> MVHLGPKKPQARKGSMADVPKELMDEIHQLEDMFTVDSETLRKVVKHFIDELNKGLTKKGGNIPMIPGWVMEFPTGKESGNYLAIDLGGTNLRVVLVKLSGNHTFDTTQSKYKLPHDMRTTKHQEELWSFIADSLKDFMVEQELLNTKDTLPLGFTFSYPASQNKINEGILQRWTKGFDIPNVEGHDVVPLLQNEISKRELPIEIVALINDTVGTLIASYYTDPETKMGVIFGTGVNGAFYDVVSDIEKLEGKLADDIPSNSPMAINCEYGSFDNEHLVLPRTKYDVAVDEQSPRPGQQAFEKMTSGYYLGELLRLVLLELNEKGLMLKDQDLSKLKQPYIMDTSYPARIEDDPFENLEDTDDIFQKDFGVKTTLPERKLIRRLCELIGTRAARLAVCGIAAICQKRGYKTGHIAADG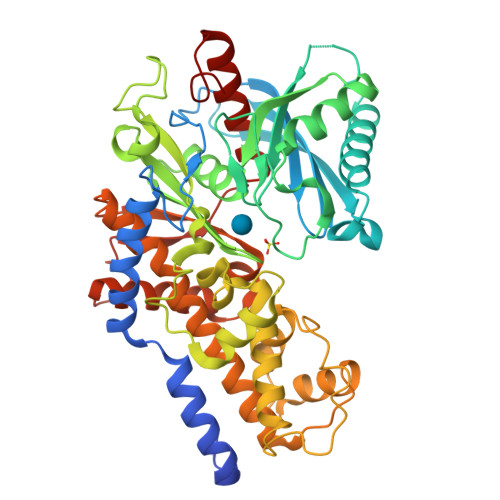SVYNKYPGFKEAAAKGLRDIYGWTGDASKDPITIVPAEDGSGAGAAVIAALSEKRIAEGKSLGIIGA>MKNFSIAKSRRLRSTPYTSRIEKQGVTAYTIYNHMLLPAAFGSIEDSYKHLKEHVQIWDVAAERQVEISGKDSAELVQLMTCRDLSKSKIGRCYYCPIIDENGNLVNDPVVLKLDENKWWISIADSDVIFFAKGLASGHKFDVKIVEPVVDIMAIQGPKSFALMEKVFGKKITELKFFGFDYFDFEGTKHLIARSGWSKQGGYEVYVENTQSGQKLYDHLFEVGKEFNVGPGCPNLIERIESALLSYGNDFDNNDNPFECGFDQYVSLDSDINFLGKEKLKEIKLKGPQKKLRGVKIDI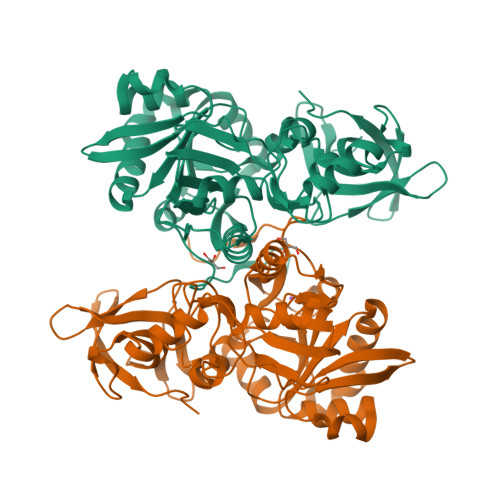KEISLTGSKNIYDENNNVIGELRSACYSPHFQKVIGIAMIKKSHWEASQGFKIQINDNTINGNVCDLPFI[2x]> 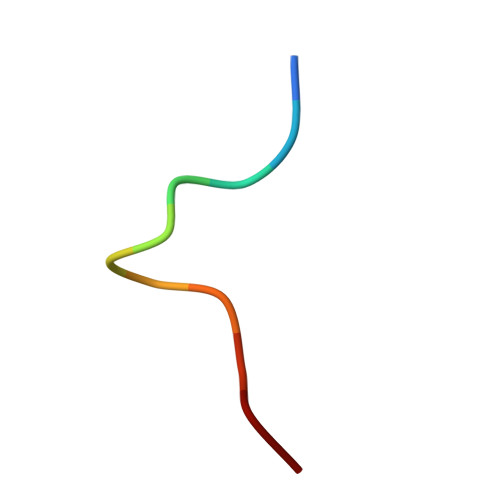LGLPDLVAKYN methyl 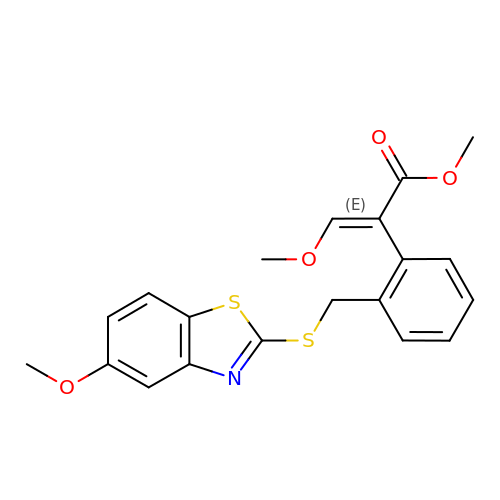(2E)-3-methoxy-2-(2-{[(5-methoxy-1,3-benzothiazol-2-yl)sulfanyl]methyl}phenyl)prop-2-enoate | C20 H19 N O4 S2 | OMGAIUZPUSZZME-LFIBNONCSA-N> MLRLSVGFLMRHIGQDVPKRHTHFVLESRLMYEKSFRDSWLHSVCRAVSQIDEPLSKTISGTRQKMLQRKVTCFQYNQYGLFKVPYYRLANVDRYHAVQGVPGTREWVPYANVSYWTMNKMVRSGNL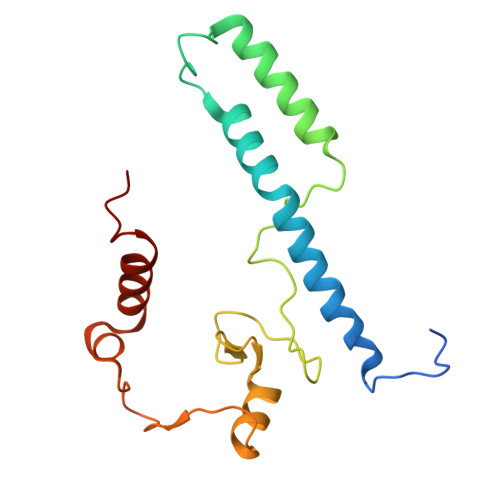LVHRVHYTGWGTDPHLKKGGWEHRWNKVMQRNALQYSRI>MHHHHHHGENLYFQGSMLTIVQEALTFDDVLLLPAYSTVLPKDVSLKTRLTRGIYLNIPLVSAAMDTVTESRMAIAMAQNGGIGILHKNMDIAAQAAEVRRVKKFEAGKAESYPNSCKDDLGRLRVGAAVGTGADTPSRVEALVEAGVDVIVVDTAHGHSAGVIERVRWVKQNFPQVQVIGGNIATGDAALALLDAGADAVKVGIGPGSICTTRIVAGIGMPQISAIDSVASALKDQIPLIADGGIRFSGDMAKAIGAGASTIMVGSLLAGTEEAPGEVEFFQGRYYKAYRGMGSLGAMAGATGSADRYFQDSKAGAEKLVPEGIEGRVPYKGPMGNIVHQMMGGLRSSMGYTGSAVIED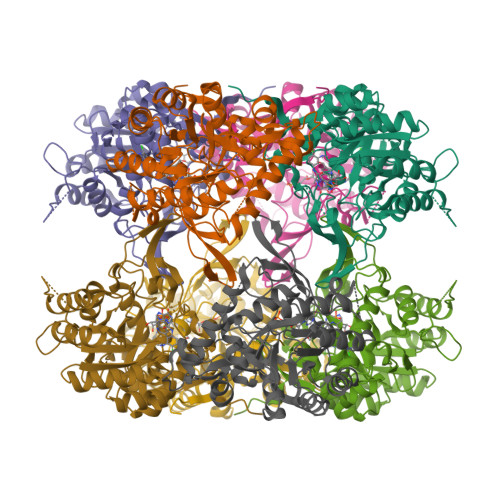LRQNAKFVKITSAGMSESHVHDVTITKEAPNYRVG[8x]>[4x]MPGSIPLIGERFPEMEVTTDHGRIKLPDHYVSQGKWFVLFSHPADFTPVCTTEFVSFARRYEDFQ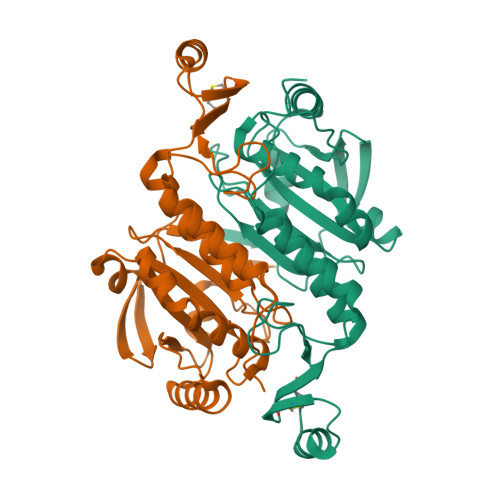RLGVDLIGLSVDSVEDHSAWKEWIERHIGVRIPFPIIADPQGTVARRLGLLHAESATHTVRGVFIVDARGVIRTMLYYPMELGRLVDEILRIVKALKLGDSLKRAVPADWPNNEIIGEGLIVPPPTTEDQARARMESGQYRCLDSWFCWDTPASRDDVEEARRYLRRAAEKPAKLLYEEARTHLH>MKHHHHHHHMHAQMTETVHKLDTNSTSQDDYVNQEELNYLNQLKDIIDHGVRKNDRTGIGTLSTFGTQSRYCLRDDIFPLLTTKRVFWRGVVEELLWFISGSTNAKQLSEKNVNIWDGNSSREFLDSRGLYNY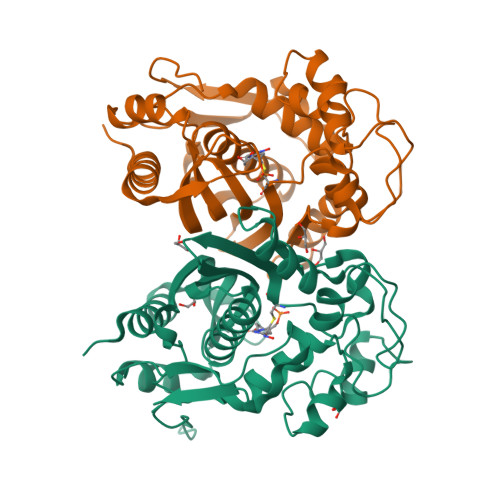EEGDLGPVYGFQWRHFGCPYSSMTADYKGKGYDQLQQCIKMIREEPESRRIIMTAWNPCDLEKVALPPCHCFVQFYVADGELSCQMYQRSADMGLGVPFNIASYSLLTRMIAHITSLKPGFFIHTIGDAHVYLTHVDALKVQMERKPRPFPKLKILRNVENIDDFRAEDFELINYKPYPKISMPMAV[2x]> AESLPDLKIEKLDEGVYVHTSFEEVNGWGVVPKHGLVVLVNAEAYLIDTPFTAKDTEKLVTWFVERGYKIKGSISSHFHSDSTGGIEWLNSRSIPTYASELTNELLKKDGKVQATNSFSGVNYWLVKNKIEVFYPGPGHTPDNVVVWLPERKILFGGCFIKPYGLGNLGDANIEAWPKSAKLLKSKYGKAKLVVPSHS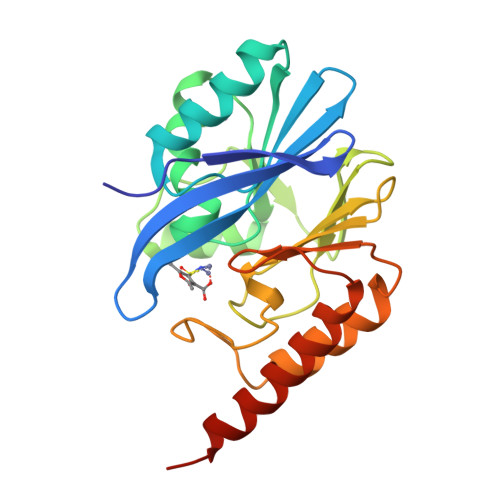EVGDASLLKLTLEQAVKGLNESKKPSKPSN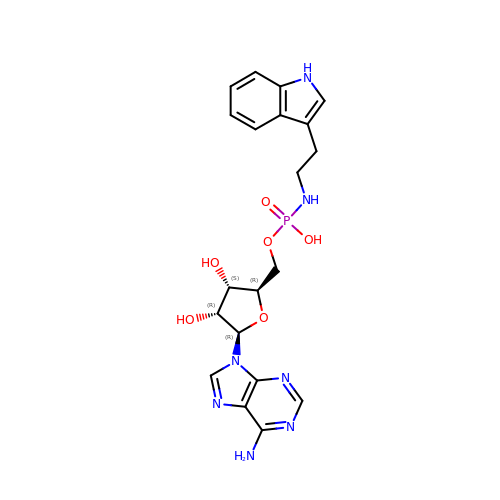[(2~{R},3~{S},4~{R},5~{R})-5-(6-aminopurin-9-yl)-3,4-bis(oxidanyl)oxolan-2-yl]methoxy-~{N}-[2-(1~{H}-indol-3-yl)ethyl]phosphonamidic acid | C20 H24 N7 O6 P | QUYHGTZYKXLUHM-WVSUBDOOSA-N> GSSHHHHHHSSGLVPRGSRRRASSLSRDAERRAYQWCREYLGGAWRRVQPEELRVYPVSGGLSNLLFRCSLPDHLPSVGEEPREVLLRLYGAILQGVDSLVLESVMFAILAERSLGPQLYGVFPEGRLEQYIPSRPLKTQELREPVLSAAIATKMAQFHGMEMPFTKEPHWLFGTMERYLKQIQDLPPTGLPEMNLLEMYSLKDEMGNLRKLLESTPSPVVFCHNDIQEGNILLLSEPENADSLMLVDFEYSSYNYRGFDIGNHFCEWVYDYTHEEWPF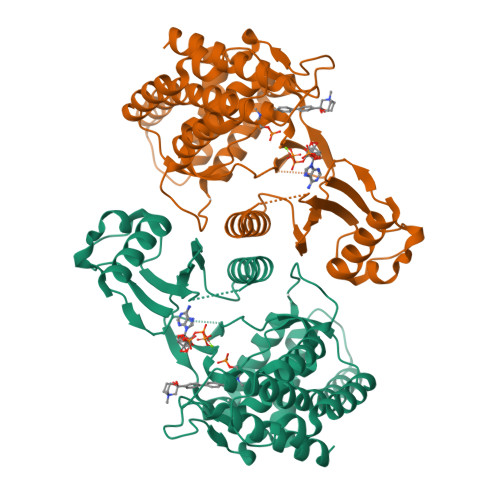YKARPTDYPTQEQQLHFIRHYLAEAKKGETLSQEEQRKLEEDLLVEVSRYALASHFFWGLWSILQASMSTIEFGYLDYAQSRFQFYFQQKGQLTSVHSSS> MMEYKIVENGLTYRIGNGASVPISNTGELIKGLRNYGPYEVPSLKYNQIALIHNNQFSSLINQLKSQISSKIDEVWHIHNINISEFIYDSPHFDSIKSQVDNAIDTGVDGIMLVLPEYNTPLYYKLKSYLINSIPSQFMRYDILSNRNLTFYVDNLLVQFVSKLGGKPWILNVDPEKGSDIIIGTGATRIDNVNLFCFAMVFKKDGTMLWNEISPIVTSSEYLTYLKSTIKKVVYGFKKSNPDWDVEKLTLHVSGK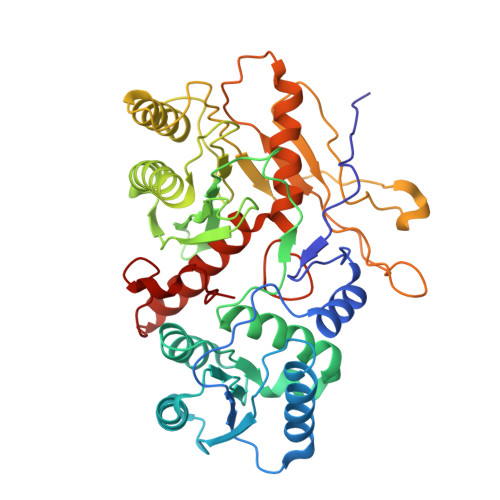RPKMKDGETKILKETVEELKKQEMVSRDVKYAILHLNETHPFWVMGDPNNRFHPYEGTKVKLSSKRYLLTLLQPYLKRNGLEMVTPIKPLSVEIVSDNWTSEEYYHNVHEILDEIYYLSKMNWRGFRSRNLPVTVNYPKLVAGIIANVNRYGGYPINPEGNRSLQTNPWFL>[12x]MRGSHHHHHHGSM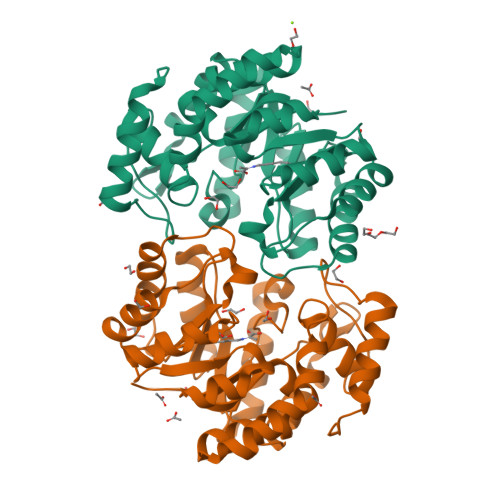DKNIIIGAMTALITPFKNGKVDEQSYARLIKRQIENGIDAVVPVGTTGESATLTHEEKRTCIEIAVETCKGTKVKVLAGAGSNATHEAVGLAKFAKEHGADGILSVAPYYNKPTQQGLYEHYKAIAQSVDIPVLLYNVPGRTGCEISTDTIIKLFRDCENIYGVKEASGNIDKCVDLLAHEPRMMLISGEDAINYPILSNGGKGVISVTSNLLPDMISALTHFALDENYKEAKKINDELYNINKILFCESNPIPIKTAMYLAGLIESLEFRLPLCSPSKENFAKIEEVMKKYKIKGF> AQDDSTPDSLFAGLVGEYYGTNSQLNNISDFRALVDSKEADATFEAANISYGRGSSDVAKGTHLQEFLGSDASTLSTDPGDNTDGGIYLQGYVYLEAG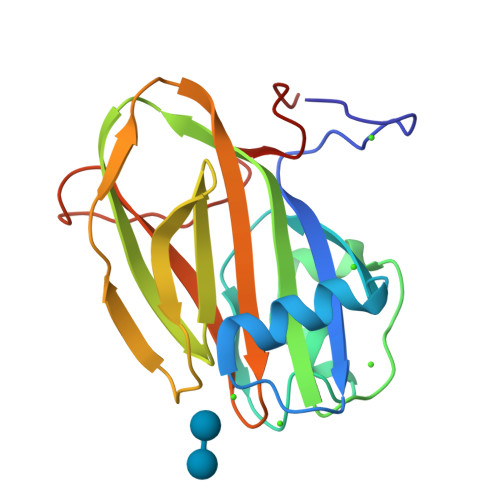TYNFKVTADDGYEITINGNPVATVDNNQSVYTVTHASFTISESGYQAIDMIWWDQGGDYVFQPTLSADGGSTYFVLDSAILSSTGETPYT> MPLEPHFMPDFLGHAENPLREEEWARLNETVIQVARRSLVGRRILDIYGPLGAGVQTVPYDEFQGVSPGAVDIVGEQETAMVFTDARKFKTIPIIYKDFLLHWRDIEAARTHNMPLDVSAAAGAAALCAQQEDELIFYGDA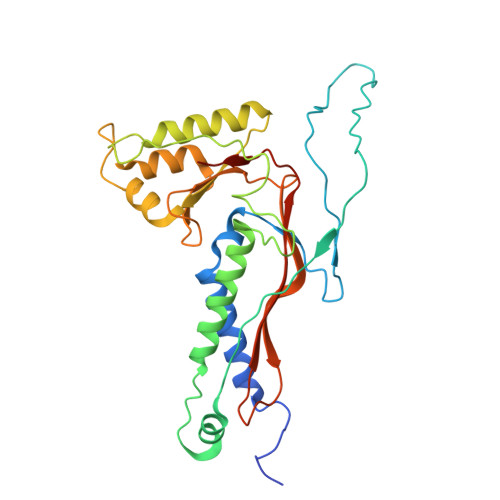RLGYEGLMTANGRLTVPLGDWTSPGGGFQAIVEATRKLNEQGHFGPYAVVLSPRLYSQLHRIYEKTGVLEIETIRQLASDGVYQSNRLRGESGVVVSTGRENMDLAVSMDMVAAYLGASRMNHPFRVLEALLLRIKHPDAICTLEGAGATERR>[4x]MRPITCSFDPVGISFQTESKQENFE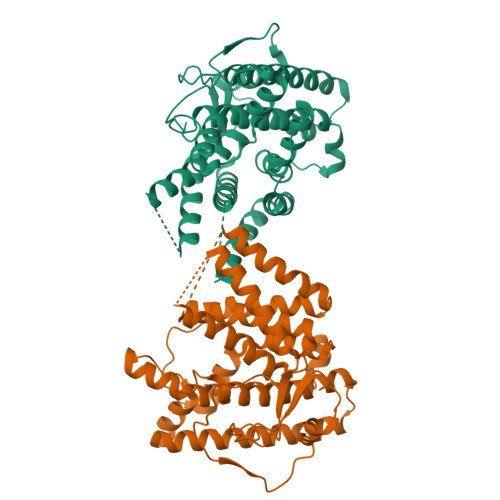FLREAISRSVPGLENCNVFDPRSLGVPWPTSFPAAAQSKYWKDAEEAAAELMDQIVAAAPGEQGSLPAELAVSDKKAAKRRELLDTSVSAPMNMFPAANAPRARIMAKAALLIFMHDDVCEYQSVQSTIIDSALADTSTPNGKGADILWQNRIFKEFSEETNREDPVVGPQFLQGILNWVEHTRKALPASMTFRSFNEYIDYRIGDFAVDFCDAAILLTCEIFLTPADMEPLRKLHRLYMTHFSLTNDLYSFNKEVVAEQETGSAVINAVRVLEQLVDTSTRSAKVLLRAFLWDLELQIHDELTRLKGTDLTPSQWRFARGMVEVCAGNIFYSATCLRYAKPGLRGI>SLRFNINDRIKELGTLIPKSNDPDMRWNKGTILKASVDYIRKLQREQQRAKELENRQKKLEHANRHLLLRIQELGIEDFLKVDLRVAKVLSAERVEGSEKLLKLTLSLGDEERTVVAGIAKYYTPEEL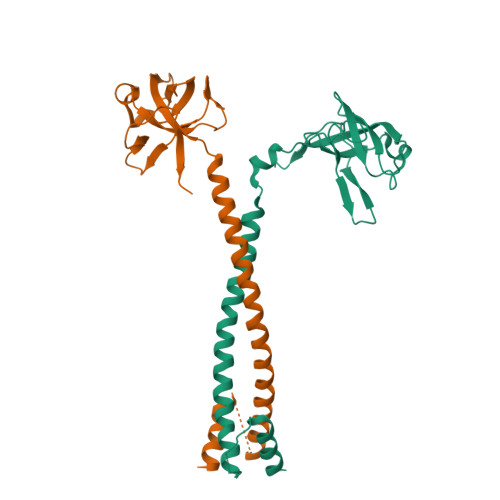VGKKIVIVANLKPRKIFGIESQGMILAASDGENLSVIVPDRDVKEGAKLSAALE[4x]>MNNQGSIISVSLGPGDPGLITVKALSQLREADVIYYPGTVSASGAVTSVALDILKEFDLDPSKLRGMLVPMSRSRGAAEASYAANYASMAEEVQAGRRVAVVSVGDGGFYSTASAIIERARRDGLDCSMTPGIPAFIAAGSAAGMPLALQSD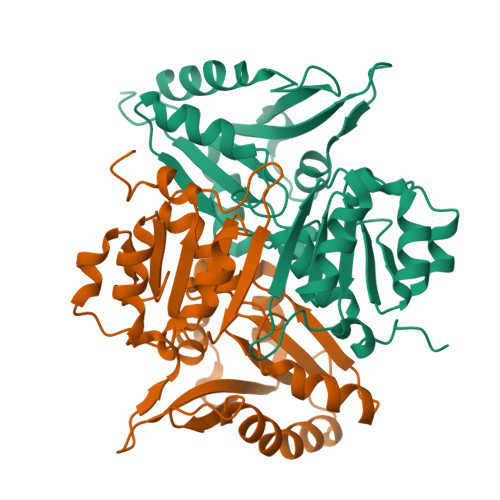SVLVLAQIDEIGELERALVTHSTVVVMKLSTVRDELVSFLERYAKPFLYAEKVGMAGEFITMEVDALRSRAIPYFSLLVCSPHCRQSTLSPFASKLAAALEHHHHHH[2x]Protein disulfide isomerase (PDI) is a major ER protein that operates as a molecular chaperone and a folding enzyme by catalyzing the formation, cleavage, and rearrangement of the disulfide bonds of unfolded or misfolded proteins. PDI consists of four tandem thioredoxin-like domains a, b, b′, and a′ plus a C-terminal extension, which are arranged into a U-shaped structure. Among the four domains, a and a′ possess a catalytic CXXC motif, which is not shared by b and b′. In particular, mutational and cross-linking analyses indicate that the b′ domain provides the principal peptide binding site in PDI16.

To determine the interaction mode of PDI with αSN, we carried out X-ray crystallographic analysis using the oxidized form of the PDI b′–a′ domains and the αSN peptide. We successfully crystallized their complex and determined the crystal structure at 1.60 Å resolution. The crystal belonged to space group P212121 with one b′–a′ molecule and one αSN peptide per asymmetric unit. Even though the two-domain arrangement was extensively affected by the crystal packing, the b′–a′ domains showed an open conformation in the oxidized state. Interestingly, the αSN undecapeptide adapts a β-hairpin structure in the crystal. Because a crystallographically neighboring molecule was accommodated in contact with the two domains, two different interaction modes were observed between the PDI b′–a′ domains and the αSN peptide. One interaction mode (termed contact-b′) was mediated through the b′ domain surface proximal to the a′ domain with a peptide-binding area of 391.6 Å2. In contact-b′, the αSN peptide was recognized through several hydrophobic interactions involving Leu38 and Val40 of αSN and Ile213, Tyr218, Met222, and Phe267 of PDI. Furthermore, the main-chain amide group of Leu38 makes a hydrogen bond with His270 Nδ1 atom. The extent of the interface area and the number of intermolecular interactions suggest that contact-b′, rather than contact-a′, primarily mediates the interaction.

> GPLGSPLIGEIGPETYSDYMSAGIPLAYIFAETAEERKELSDKLKPIAEAQRGVINFGTIDAKAFGAHAGNLNLKTDKFPAFAIQEVAKNQKFPFDQEKEITFEAIKAFVDDFVAGKIEPSIKSEPIPEKQEGPVTVVVAKNYNEIVLDDTKDVLIEFYAPWCGHCKALAPKYEELGALYAKSEFKDRVVIAKVDATANDVPDEIQGFPTIKLYPAGAKGQPVTYSGSRTVEDLIKFIAENGKYKAA;> GKTKEGVLYVG>SMQQRKVLTLEKEDNQTFGFEIQTYGLHHREEQRVEMVTFVCRVHESSPAQLAGLTPGDTIASVNGLNVEGIRHREIVDIIKASGN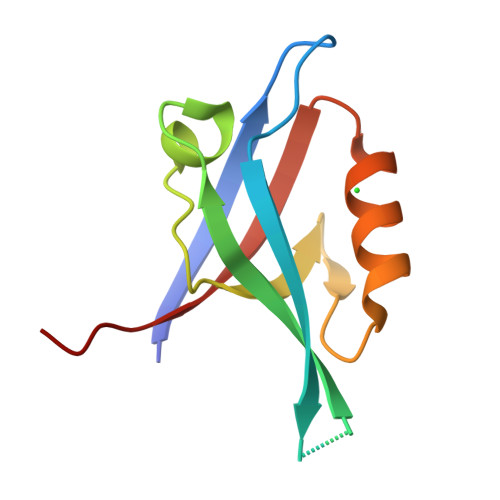VLRLETLYSSTL[2x]> SNASIVSLLGIKVLNNPAKFTDPYEFEITFECLESLKHDLEWKLTYVGSSRSLDHDQELDSILVGPVPVGVNKFVFSADPPSAELIPASELVSVTVILLSCSYDGREFVRVGYYVNNEYDEEELRENPPAKVQVDHIVRNILAEKPRVTRFNIVWDNAAGAATAAKKEIKLARRLRGER

The histone H3/H4 chaperone Asf1 (anti-silencing function 1) is required for the establishment and maintenance of proper chromatin structure, as well as for genome stability in eukaryotes. Asf1 is the common entity shared by the RC and RI pathways, because it binds to and stimulates histone deposition by both the CAF-1 and HIR complexes. Asf1 proteins from all eukaryotes share a very conserved 155 residue N-terminal immunoglobulin-like fold domain. Asf1 alone adopts a switched-type immunoglobulin-like (Ig-like) fold containing two extra, short β-strands (termed h and h').

We determined the structure of the conserved N-terminus of budding yeast Asf1 bound to the C-terminal α3 helix of yeast histone H3 to 2.2 Å resolution. Because the interaction between the C-terminal histone H3 α3 helix (H3α3) and Asf1 is of modest affinity (micromolar Kd), we stabilized the association by fusing Asf1N to H3α3 with a flexible linker peptide. The global fold of Asf1N in the current structure is nearly identical to that solved previously without the histone helix. The only significant changes in the structure are a forward rotation of the loop connecting β-strands c and c', as well as a small rotation of the loop and α-helix connecting β-strands e and f. The structure solved here shows that the histone helix binds to Asf1 in this predicted region, but in an unanticipated orientation. The H3 α-helix lies in a pocket defined by hydrophobic residues on one side and an intricate hydrogen-bonding network on the other. Notably, to properly form the pocket, the β-c/β-c' connecting loop folds downward (as compared to the structure of unbound yeast Asf1N), bringing residues Ser48 and Ser50 in proximity to contribute to the hydrogen-bonding network ("loop 1" in Figure 1B). Leu130 makes van der Waals contacts to Asf1 amino acids Val94, Tyr112, Arg145, and Leu96. A lone salt bridge is formed between the invariant residues Asp54 on Asf1 and Arg129 on H3. By binding to and occluding proper formation of the four-helix bundle, Asf1 is positioned to directly disrupt histone tetramerization.> APADPVPTVFFGDSYTANFGIAPVTNQDSERGWCFQAKENYPAVATRSLADKGITLDVQADVSCGGALIHHFWEKQELPFGAGELPPQQDALKQDTQLTVGSLGGNTLGFNRILKQCSDELRKPSLLPGDPVDGDEPAAKCGEFFGTGDGKQWLDDQFERV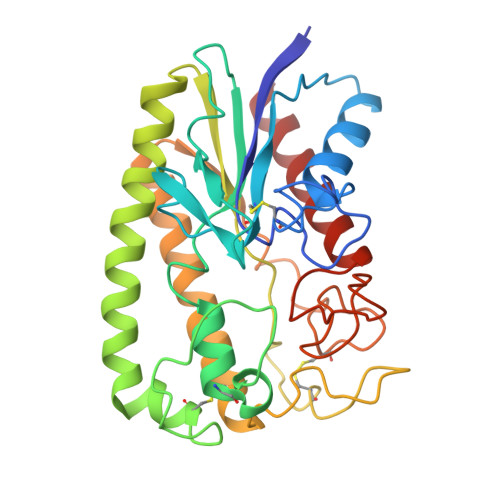GAELEELLDRIGYFAPDAKRVLVGYPRLVPEDTTKCLTAAPGQTQLPFADIPQDALPVLDQIQKRLNDAMKKAAADGGADFVDLYAGTGANTACDGADRGIGGLLEDSQLELLGTKIPWYAHPNDKGRDIQAKQVADKIEEILNR>MKYILVTGGVISGVGKGVIASSFGTLLKSCGLDVTSIKIDPYINIDAGTFSPYEHGEVYVLDDGAEVDLDLGNYERFLDVTLHRDNNITTGKIYKLVIEKERTGEYLGKTVQVVPHITDAIQEWVERVAQTPVQGSSKPQVCIVELGGTIGDIEGMPFVEAFRQFQFRVKRENFCLAHVSLVPLPKATGEPKTKPTQSSVRELRGCGLSPDLIVCRSEKPIGLEVKEKISNFCHVGPDQVICIHDLNSIYHVPLLMEQNGVIEYLNERLQLNIDMSKRTKCLQQWRDLARRTETVRREVCIAVVGKYTKFTDSYASVVKALQHAALAVNRKLELVFIESCLLEEETLHSEPSKYHKEWQKLCDSHGILVPGGFGSRGMEGKIRACQWARENQKPLLGICLGLQAAVIEFARNKLGLKDANTTEIDPNTANALVIDMPEHHTGQLGGTMRLGKRITVFSDGPSVIRQLYGNPKSVQERHRHRYEVNPKYVHLLEEQGMRFVGTDVDKTRMEIIELSGHPYFVATQYHPEYLSRPLKPSPPFLGLILASVDRLNQYIQ[4x]

Cytidine triphosphate synthase (CTPS) catalyzes the final and rate-limiting step of de novo CTP biosynthesis, in which a UTP is converted into CTP with the consumption of an ATP and a glutamine. A CTPS protein comprises two domains, the N-terminal ammonia ligase (AL) domain and the C-terminal glutamine amidotransferase (GAT) domain. While the active site at the AL domain activates UTP by phosphorylation using ATP to generate an iminophosphate intermediate that can react with ammonia to yield CTP, the GAT domain mediates the hydrolysis of glutamine to yield NH3 with GTP as allosteric activator. The nascent ammonia is delivered through an “ammonia tunnel,” which connects the active sites at both domains, to complete the reaction.

For the product-bound state (dmCTPS+Pro), we imaged dmCTPS in the presence of 10 mM Mg2+ and 2 mM CTP and picked 1,563,553 particles. In contrast, the dmCTPS+Pro model represents an inhibited state of dmCTPS. In this conformation, the UTP binding site is occupied by CTP as a well-known competitive inhibitor. To our surprise, we identified a second CTP molecule in an individual subunit of the dmCTPS+Pro tetramer, whose binding site overlaps with ATP/ADP. Since CTP is the only nucleotide present under the conditions of analysis, it is unlikely that another molecule could be mistaken for CTP in our map. In addition, the electron density agrees very well with the CTP structure, confirming our findings of the CTP binding site of CTPS and also raising the possibility that binding competition, which inhibits the activity of CTPS, may occur at both the UTP and ATP binding sites. However, the unexpected finding of a CTP molecule siting at the ATP/ADP binding site of the map gives rise to the notion that CTP may block CTPS by competing with UTP and also with ATP, suggesting an added level of complexity of feedback inhibition. The wing is also flexible in our dmCTPS+Pro model. In the dmCTPS+Pro tetramer, the length is around 23.5 Å, and the diameter ranges from 3.38 to 5.54 Å. We analyzed the conformational change at the UTP binding site and determined that the distance from CTP to the exit of the tunnel is about 18.8 Å in the dmCTPS+Pro, whereas UTP in dmCTPS+Sub sits right before the opening at a distance of about 5.4 Å.>GPMGKPARKGAEWKRFLKNNWVLLSTVAAVVLGITTGVLVREHSNLSTLEKFYFAFPGEILMRMLKLIILPLIISSMITGVAALDSNVSGKIGLRAVVYYFATTLIAVILGIVLVVSIKPGVTQKVGEIARTGSTPEVSTVDAMLDLIRNMFPENLVQAAFQQYKTKREEVKPPSDPEMTMTEESFTAVMTTAISKTKTKEYKIVGMYSDGINVLGLIVFALVFGLVIGKMGEKGQILVDFFNALSDATMKIVQIIMWYMPLGILFLIAGCIIEVEDWEIFRKLGLYMATVLTGLAIHSIVILPLIYFIVVRKNPFRFAMGMAQALLTALMISSSSATLPVTFRCAEENNQVDKRITRFVLPVGATINMDGTALYEAVAAVFIAQLNDLDLGIGQIITISITATSASIGAAGVPQAGLVTMVIVLSAVGLPAEDVTLIIAVDCLLDRFRTMVNVLGDAFGTGIVEKLSKKELEQMDVSSEVNIVNPFALESTILDNEDSDTKKSYVNGGFAVDKSDTISFTQTSQF[3x]

Human excitatory amino acid transporters (EAATs) concentrate the neurotransmitter glutamate and aspartate in cells. By coupling the uptake of one substrate molecule to movements of five ions—symport of three sodium (Na+) ions and a proton and countertransport of one potassium (K+) ion—EAATs ensure that the cytoplasmic glutamate concentration is ~10 mM, which is required for neuronal functions, while the extracellular concentrations are as low as a few nM permitting rounds of synaptic signaling. EAATs are homotrimers composed of promoters that work independently. TMs 1, 2, 4, and 5 of each protomer comprise the scaffold domain mediating trimerization; TMs 3, 6, 7, and 8 and helical hairpins (HPs) 1 and 2 form the substrate-binding transport domain.

EAAT3-X was predominantly found in OFS in NaCl buffer and iOFS in NMDG, NaCl/glutamate, and KCl buffers. In contrast to iOFS-Na+, OFS-Na+ shows wide-open HP2 and a fully solvent-exposed substrate-binding site. R447 interacts with Y373, already in place for glutamate coordination. In contrast, in OFS-Apo and OFS-Na+, E374 is buried and proximal to G415. It is likely protonated with pKa-s of 9.2, 10.0, and 7.6 for OFS-ApoK, OFS-ApoNMDG, and OFS-Na+, respectively. In contrast, OFS-Na+ and OFS-Apo feature fully open HP2-s, and only transmitter binding can close the gate. hEAAT3g in the IFS, bound to Na+ ions or apo, also pictures an open HP2. Na+ ions bind with high affinity to OFS-Apo, and OFS-Na+ might be the resting state in cells under physiologic conditions. The neurotransmitter and Na2 bind to OFS-Na+, promoting HP2 closure and transition into iOFS*-Glu and IFS-Glu.>QPVRYSIPEELDRGSVVGKLAKDLGLSVLEVSARKLRVSAEKLHFSVDSESGDLLVKDRIDREQICKGRRKCELQLEAVLENPLNIFHVVVEIEDVNDHAPQFPKDEINLEISESDSPGARTILESAKDLDIGMNSLSKYQLSPNDYFLLLVKDNPDGSKYPELELQKMLDREAESTHHLMLTAVDGGDPPRTGTTQLRIRVVDANDNRPVFSQDVYRVRLPEDLPPGTTVLRLKAMDQDEGINAEFTYSFLGVANKAQFSLDPITGDIVTRQSLDFEEVEQYTIDVEAKDRGSLSSQCKVIIEVLDENDNRPEIIITSLSDQISEDSPSGTVVALFKVRDRDSGENAEVMCSLSGNNPFKIHSSSNNYYKLVTDSILDREQTPGYNVTITATDRGKPPLSSSTTITLNVADVNDHHHHHHHH[2x]

By contrast, in vertebrates the clustered protocadherins (Pcdhs) provide analogous cell-surface diversity, but in this case generated through stochastic alternative promoter choice. Biophysical measurements with domain-deleted proteins showed that Pcdhs also interact in cis, through a membrane-proximal dimer interface involving extracellular cadherin domain 6 (EC6) and potentially EC5. The specificity-determining cell-cell recognition interface of Pcdhs involves domains EC1–4, as shown experimentally through mutagenesis analysis and suggested by mutation correlation analysis.

Crystallization screening of these dimeric γ-Pcdh fragments yielded crystals of γA1EC1–4, γA8EC1–4, γA9EC1–5, γB2EC1–5, and γB7EC1–4, and their structures were determined by molecular replacement. X-ray diffraction by the γA9EC1–5 and γB7EC1–4 crystal form 1 crystals was significantly anisotropic and therefore the data was truncated using ellipsoidal limits for structure determination and refinement (Figure 1—source data 1 and Figure 1—figure supplement 2). The resolution of the final refined structures was 4.2 Å for γA1EC1–4, 3.6 Å for γA8EC1–4, 2.9/4.3/3.2 Å for γA9EC1–5, 3.5 Å for γB2EC1–5, 4.5/4.5/3.6 Å for γB7EC1–4 crystal form 1, and 3.1 Å for γB7EC1–4 crystal form 2. The γB2EC1–5 and γB7EC1–4trans dimer structures show the same overall arrangement as the previously published γB3EC1–4 trans dimer structure. The γB7 structure reveals a salt bridge in the EC1:EC4 interface between residues E41 in EC1 and K338 in EC4. Both E41 and K338 are conserved in all γB isoforms so that this salt bridge is likely present in all γB homodimers. In addition, residue R340, which is also conserved in all γB isoforms, is positioned so that it could form an additional salt bridge with E41. Thus, a putative heterodimer formed between any γB isoform and any γA isoform would position a positively charged residue at position 41 in the EC1 domain of the γA isoform in close proximity to K338 and R340 in the γB isoform, which would significantly weaken binding.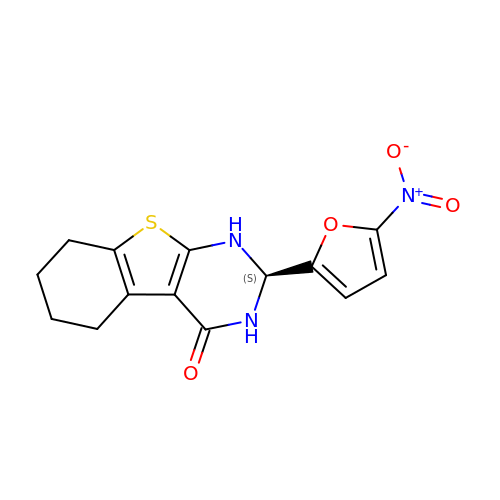(2~{S})-2-(5-nitrofuran-2-yl)-2,3,5,6,7,8-hexahydro-1~{H}-[1]benzothiolo[2,3-d]pyrimidin-4-one | C14 H13 N3 O4 S | MOKSPNCNIWVHBB-LBPRGKRZSA-N>MATGSGSLIWFRKGLRVHDNPALEYASKGSEFMYPVFVIDPHYMESDPSAFSPGSSRAGVNRIRFLLESLKDLDSSLKKLGSRLLVFKGEPGEVLVRCLQEWKVKRLCFEYDTDPYYQALDVKVKDYASSTGVEVFSPVSHTLFNPAHIIEKNGGKPPLSYQSFLKVAGEPSCAKSELVMSYSSLPPIGDIGNLGISEVPSLEELGYKDDEQADWTPFRGGESEALKRLTKSISDKAWVANFEKPKGDPSAFLKPATTVMSPYLKFGCLSSRYFYQCLQNIYKDVKKHTSPPVSLLGQLLWREFFYTTAFGTPNFDKMKGNRICKQIPWNEDHAMLAAWRDGKTGYPWIDAIMVQLLKWGWMHHLARHCVACFLTRGDLFIHWEQGRDVFERLLIDSDWAINNGNWMWL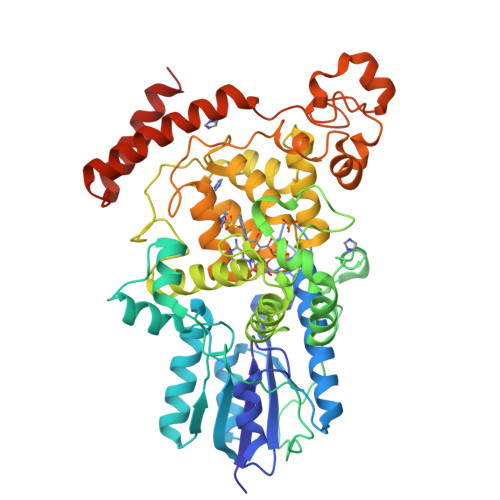SCSSFFYQFNRIYSPISFGKKYDPDGKYIRHFLPVLKDMPKQYIYEPWTAPLSVQTKANCIVGKDYPKPMVLHDSASKECKRKMGEAYALNKKMDGKVDEENLRDLRRKLQKDEHEESKIRNQRPKLK[3x]CYCLO-(L-TYROSINE-L-PROLINE) INHIBITOR | C14 H16 N2 O3 | 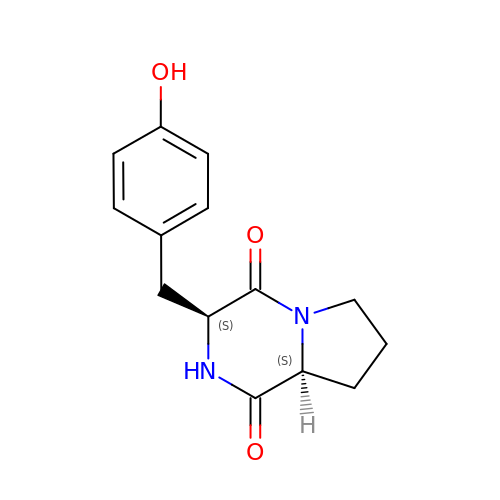LSGOTAXPWMCUCK-RYUDHWBXSA-N>[2x]ILEGRECIPHSQPWQAALFQGERLICGGVLVGDRWVLTAAHCKKQKYSVRLGDHSLQSRDQPEQEIQVAQSIQHPCYNNSNPEDH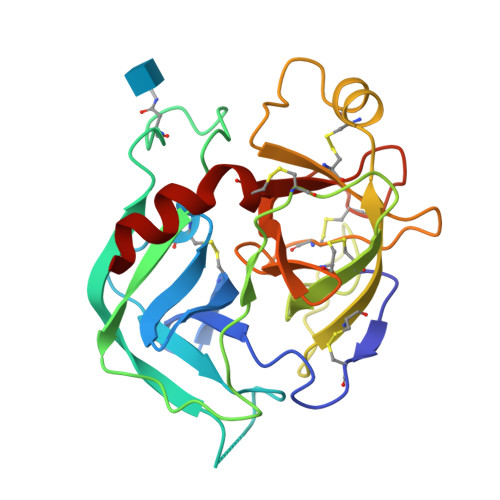SHDIMLIRLQNSANLGDKVKPVQLANLCPKVGQKCIISGWGTVTSPQENFPNTLNCAEVKIYSQNKCERAYPGKITEGMVCAGSSNGADTCQGDSGGPLVCDGMLQGITSWGSDPCGKPEKPGVYTKICRYTTWIKKTMD> MGLLTILKKMKQKERELRLLMLGLDNAGKTTILKKFNGEDIDTISPTLGFNIKTLEHRGFKLNIWDVGGQKSLRSYWRNYFESTDGLIWVVDSADRQRMQDCQRELQSLLVEERLAGATLLIFANKQDLPGALSSNAIREVLELDSIRSHHWCIQGCSAVTGENLLPGIDWLLDDISSRIFTADLEHHHHHH;> GSMDALEGESFALSFSSASDAEFDAVVGYLEDIIMDDEFQLLQRNFMDKYY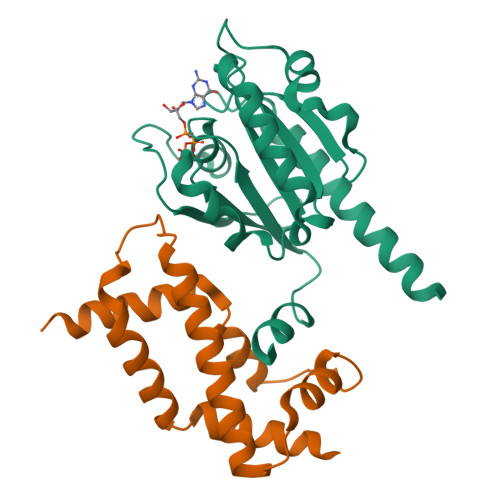LEFEDTEENKLIYTPIFNEYISLVEKYIEEQLLQRIPEFNMAAFTTTLQHHKDEVAGDIFDMLLTFTDFLAFKEMFLDYRAEKEGRGLDLSSGLVVTSLCKSSSLPASQNNLRH>[8x]MNLPTAQEVQGLMARYIELVD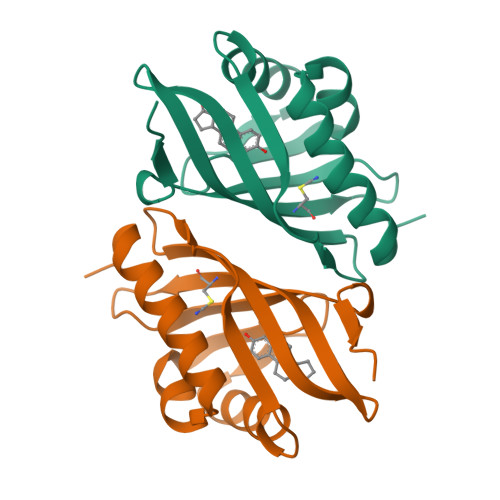VGDIEAIVQMYADDATVENPFGQPPIHGREQIAAFYRQGLGGGKVRASLTGPVRASHNGSGAMPFRVEMVWNGQPSALDVIDVCRFDEHGRIQTMQAYWSEVNLSVREPQ>[2x]MAIPAFHPGELNVYSAPGDVADVSRALRLTGRRVMLVPTMGALHEGHLALVRAAKRVPGSVVVVSIFVNPMQFGAGGDLDAYPRTPDDDLAQLRAEGVEIAFTPTTAAMYPDGLRTTVQPGPLAAELEGGPRPTHFAGVLTVVLKLLQIVRPDRVFFGEKDYQQLVLIRQLVADFNLDVAVVGVPTVREADGLAMSSRNRYLDPAQRAA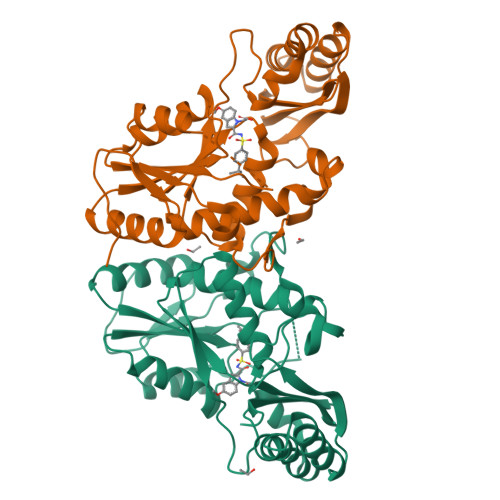AVALSAALTAAAHAATAGAQAALDAARAVLDAAPGVAVDYLELRDIGLGPMPLNGSGRLLVAARLGTTRLLDNIAIEIGTFAGTDRPDGYR> KPYEKVRIYRMDGSYRSVELKHGNNTTVQQIMEGMRLSQETQQYFTIWICSENLSLQLKPYHKPLQHVRDWPEILAELTNLDPQRETPQLFLRRDVRLPLEVEKQIEDPLAILILFDEARYNLLKGFYTAPDAKLITLASLLLQIVYGNYESKKHKQGFLNEENLKSIVPVTKLKSKAPHWTNRILHEYKNLSTSEGVSKEMHHLQRMFLQNCWEIPTYGAAFFTGQIFTKASPSNHKVIPVYVGVNIKGLHLLNMETKALLISLKYGCFMWQLGDTDTCFQIHSMENKMSFIVHTKQAGLVVKLLMKLNGQLMPTERNS;> MREYKLVVLGSGGVGKSALTVQFVQGIFVEKYDPTIEDSYRKQVEVDAQQCMLEILDTAGTEQFTAMRDLYMKNGQGFALVYSITAQSTFNDLQDLREQILRVKDTDDVPMILVGNKCDLEDERVVGKEQGQNLARQWNNCAFLESSAKSKINVNEIFYDLVRQINR

Herein, we characterize the 2-hydroxy-1-naphthaldehyde (HNA) fragment as a targeted covalent reversible ligand of a noncatalytic lysine (Lys720) of the Krev interaction trapped 1 (KRIT1) protein. The PPI between HEG1 and KRIT1 is believed to play an important role in controlling vascular development and permeability under normal and pathological conditions. The HEG1 binding domain of KRIT1 features three lysines, namely Lys475, Lys720, and Lys724; based on point mutation studies, these residues are essential for the interaction between HEG1 and KRIT1.14 The HNA was found to form a reversible imine adduct with Lys720, and SAR studies indicated that the HNA is the smallest/simplest 2-hydroxy-arylaldehyde that inhibits the HEG1-KRIT1 PPI. However, the interaction of HNA within the HEG1 binding pocket of KRIT1 induces proximity of the aldehyde moiety with the ε-amino group of Lys720, resulting in the specific targeting of this amino acid residue.

To evaluate the potential of the HNA as a site-directing fragment to identify HEG1-KRIT1 PPI inhibitors with potentially improved binding affinity and inhibition activity, we synthesized and screened a series of HNA derivatives bearing substitutions at the C6 or C7 position of the naphthalene ring. The C6 and C7 positions were selected for substitutions as an analysis of the available HNA-KRIT1 co-crystal structure indicated that these two positions may provide opportunities for analogs with improved complementarity to the HEG1 binding region of KRIT1. The co-crystal structures of 3, 5, and 6 in complex with KRIT1 revealed that these compounds exhibit similar binding modes as the parent HNA fragment, including the presence of the imine adduct between the aldehyde moiety of the HNA derivative and the ε-amino group of Lys720. However, compared to the unsubstituted HNA, derivatives 3, 5, and 6 established additional interactions with KRIT1. Additionally, both furan derivatives 5 and 6 were involved in hydrogen−π interactions with KRIT1 Gln473. Interestingly, the binding positions in the three crystal structures appeared nearly identical with the HNA binding pose generated in the MD simulations. Thus, the X-ray and activity data indicate that the binding affinity of the HNA for KRIT1, and the consequent inhibition activity of this fragment in the HEG1–KRIT1 PPI assay, respond to elements of SARs, and in turn highlight the importance of structure complementarity and templating effects in promoting the formation of specific and relatively stable imine adducts with KRIT1 Lys720.>[2x]MPPVSSARNLKELPKFRDGLSYLYVEHAVVEREAGGIGIYDQEGLTLAPVAGLGVLFLGPGTRITHAAVRLLAENGCTVAWVGEGMARFYAQGLGDTRSAARFYRQARAWADPALHLEVVMRLYRMRFSEPLPEGLTLEQVRGLEGVRVRNAYARWSRETGVPWYGRSYDRGNWRAADPVNRALSAGASYLYGLAHAAIVSLGFSPALGFIHTGK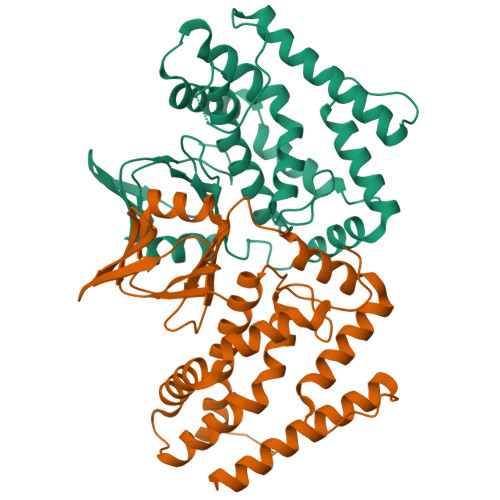LLSFVYDIADLYKADYLVPAAFRTVAESEEAVERRVRRALREAIQEGRLLERMAEDLLNLFRGLGLPEEEDPVEEDPTRPGGLWDLEGEVEGGVAYGGDDPGEGAEEPEG>[2x]MDYKDDDDKGSSTSLYKKAGSETLYIQGQDEYYMARALKLAQRGRFTTHPNPNVGCVIVKDGEIVGEGYHQRAGEPHAEVHALRMAGEKAKGATAYVTLEPCSHHGRTPPCCDALIAAGVARVVASMQDPNPQVAGRGLYRL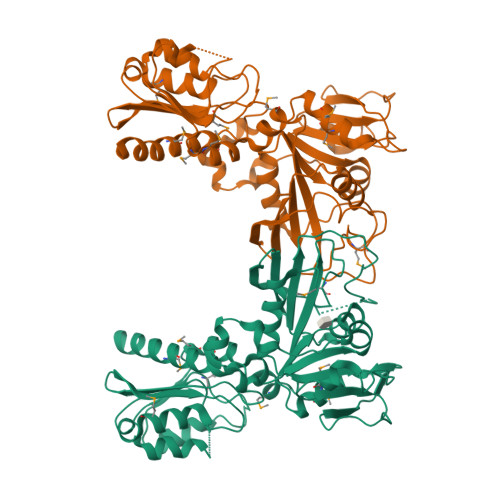QQAGIDVSHGLMMSEAEQLNKGFLKRMRTGFPYIQLKLGASLDGRTAMASGESQWITSPQARRDVQLLRAQSHAILTSSATVLADDPALTVRWSELDEQTQALYPQQNLRQPIRIVIDSQNRVTPVHRIVQQPGETWFARTQEDSREWPETVRTLLIPEHKGHLDLVVLMMQLGKQQINSIWVEAGPTLAGALLQAGLVDELIVYIAPKLLGSDARGLCTLPGLEKLADAPQFKFKEIRHVGPDVCLHLVGASTHHHHHH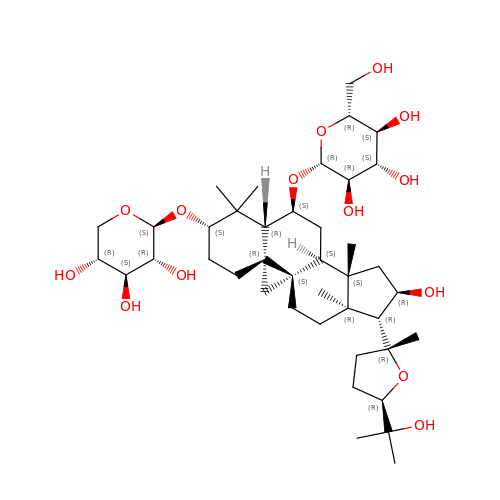Astragaloside IV | C41 H68 O14 | QMNWISYXSJWHRY-RDWDXCDVSA-N>MSNSKFNVRLLTEIAFMAALAFIISLIPNTVYGWIIVEIACIPILLLSLRRGLTAGLVGGLIWGILSMITGHAYILSLSQAFLEYLVAPVSLGIAGLFRQKTAPLKLAPVLLGTFVAVLLKYFFHFIAGIIFWSQYAWKGWGAVAYSLAVNGISGILTAIAAFVILIIFVKKFPKLFIHS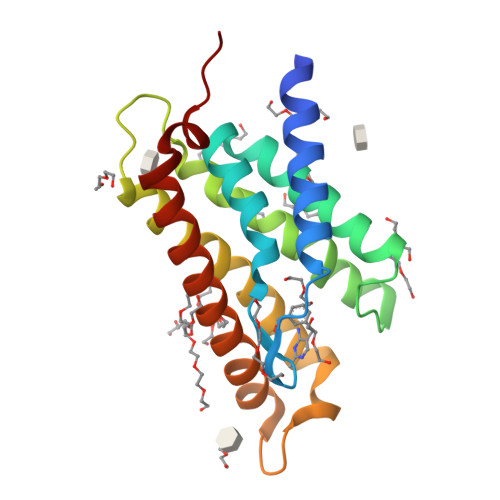NY[2x]> MSVSSLLEVVADDLLKLNNNLKSLVGAENPVLVSAAEQIFGAGGKRLRPALVFLVSRATAELAGLLELTTEHQRLAEIIEMIHTASLIHDDVIDDSGMRRGKETIHQLYGTRVAVLAGDFMFAQSSWFLANLENIEVIKLISQVIKDFASGEIKQASTLFDCDITLDDYLLKSYYKTASLIAASTRSAAIFSGVSTAICEQMYEYGRNLGLSFQVVDDILDFTQSAEQLGKPAGSDLAKGNLTAPVIFALQDEPQLREIIDSEFS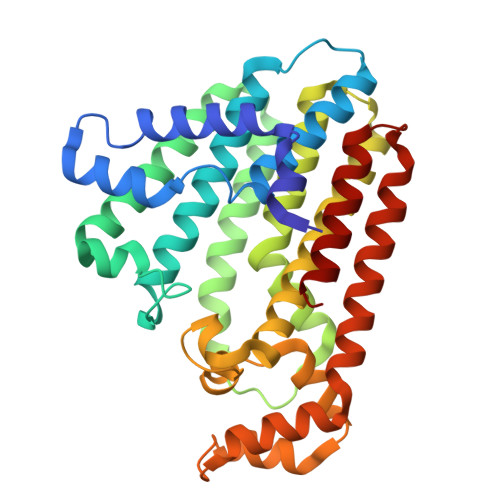ETNSLATAIELVHRSGGIKRAHELAREKGEIAIQSLQCLPRSEFRSTLENMVKYNLERID~{N}-(2-chloranyl-6-methyl-phenyl)-2-[[3-[[(3~{R},4~{R})-3-fluoranylpiperidin-4-yl]carbamoyl]phenyl]amino]-1,3-thiazole-5-carboxamide 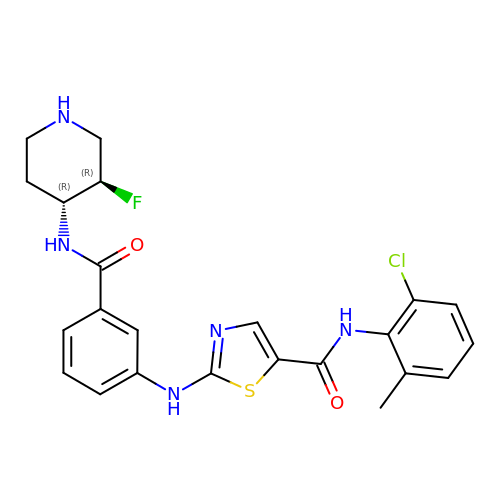| C23 H23 Cl F N5 O2 S | RRUBGRARVNLPQT-QZTJIDSGSA-N> MWVYRLKGTLEALDPILPGLFDGGARGLWEREGEVWAFFPAPVDLPYEGVWEEVGDEDWLEAWRRDLKPALAPPFVVLAPWHTWEGAEIPLVIEPGMAFGTGHHETTRLALKALARHLRPGDKVLDLGTGSGVLAIAAEKLGGKALGVDIDPM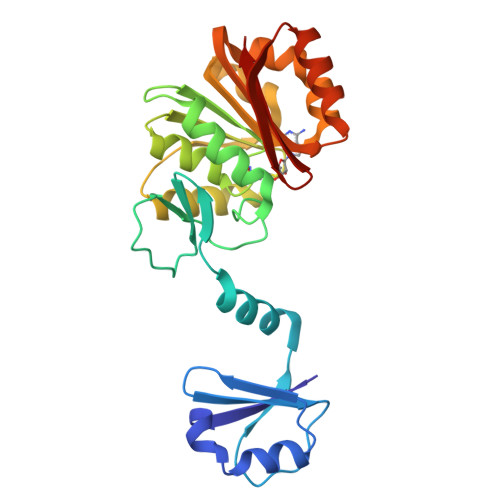VLPQAEANAKRNGVRPRFLEGSLEAALPFGPFDLLVANLYAELHAALAPRYREALVPGGRALLTGILKDRAPLVREAMAGAGFRPLEEAAEGEWVLLAYGR(2Z)-3-(4-fluorophenyl)-2-sulfanylprop-2-enoic acid | C9 H7 F O2 S | 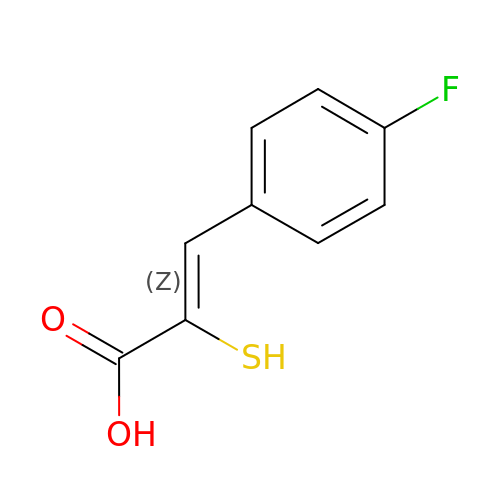IBSBBUUSPOCCFV-YVMONPNESA-N> MIMSKIAETAKRLADSLRELRRILEELKEMLERLEKRPDKKVIVDVLKVIVKAIEASVENQRISASNQAALALAIAAEAVKEIEEDIDRARKLKDEGNKEEAEKVLRKAREKIREVRDALDAIAKGAGTPDIALKAAELLVRLIKLLIEIAKLLQDAGNKEEAEKVLREATELIKRVTELLEKIAKNSDTPELALRAAELLVRLIKLLIEIAKLLQEQGNKEEAEKVLREATKMIIRVAQLLVKIA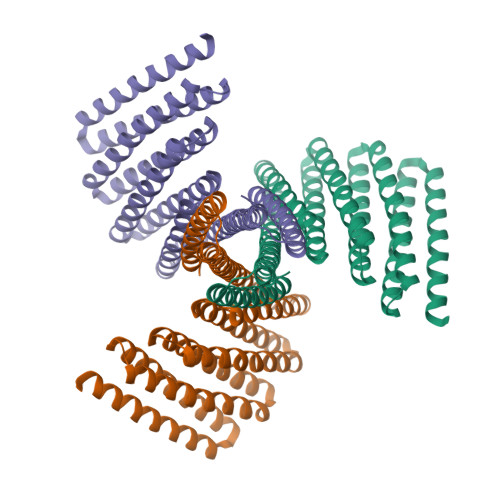KNSDEPELAKRAAELLKRLIELLKEIAKLLEEEGNEDEAEKVKEIAKILEEAVRELEERIIGGSWSGGGSEQKLISEEDLGGS>MVRIYTLTLAPSLDSATITPQIYPEGKLRCTAPVFEPGGGGINVARAIAHLGGSATAIFPAGGATGEHLVSLLADENVPVATVEAKDWTRQNLHVHVEASGEQYRFVMPGAALNEDEFRQLEEQVLEIESGAILVISGSLPPGVKLEKLTQLISAAQKQGIRCIVDSSGEALSAALAIGNIELVKPNQKELSALVNRELTQPDDVRKAAQEIVNSGKAKRVVVSLGPQGALGVDSENCIQVVPPPVKSQSTVGAGDSMVGAMTLKLAENASLEEMVRFGVAAGSAATLNQGT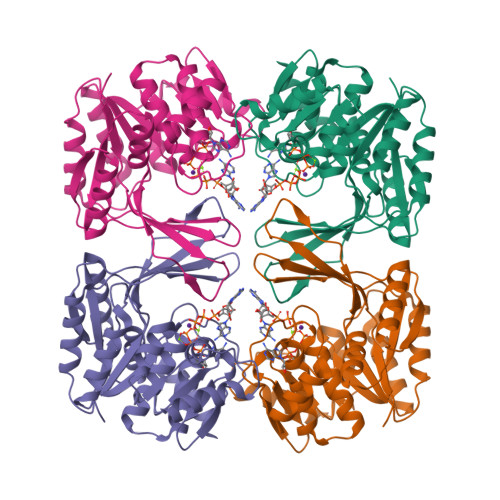RLCSHDDTQKIYAYLSR[2x]>[2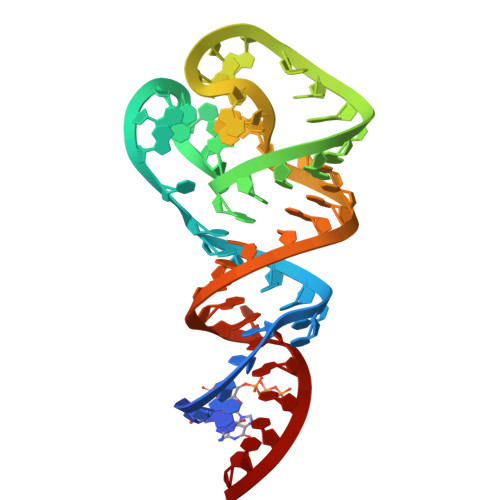x]GGAACCCUCUCUUCCGAAGCGAGCCGGGGGCGGUGGGAGCCCGGUGAAGACGGUUCC> SLAKRIIAALEVKDGRVVKGTNFENLRDSGDPAELGKFYSEIGIDELVFHDHTASVEKRKTMLELVEKVAEQIDIPFTVGGGIHDFETASELILRGADKVSINTAAVENPSLITQIAQ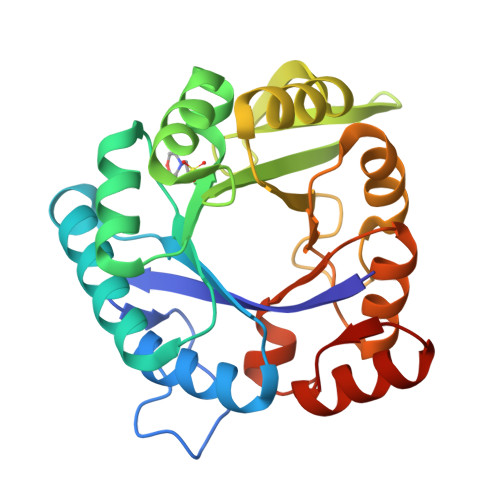TFGSQAVVVAIDAKRVDGEFMVFTYSGKKNTGILLRDWVVEVEKRGAGEILLTSIDRDGTKSGYDTEMIRFVRPLTTLPIIASGGAGKMEHFLEAFLAGADAALAASVFHFREIDVRELKEYLKKHGVNVRLEGL> VIRVYIASSSGSTAIKKKQQDVLGFLEANKIGFEEKDIAANEENRKWMRENV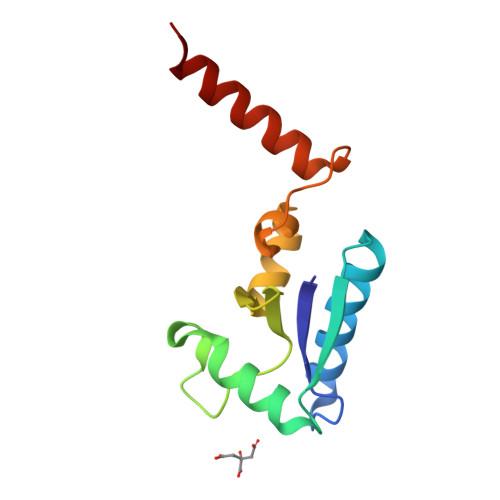PENSRPATGYPLPPQIFNESQYRGDYDAFFEARENNAVYAFLGLTAPPGSKEAEVQAKQQALEHHHHHH> ASLGHPATFGRATHVVVRALPESLAQQALRRTKGDEVDFARAERQHQLYVGVLGSKLGLQVVQLPADESLPDCVFVEDVAVVCEETALITRPGAPSRRKEADMMKEALEKLQLNIVEMKDENATLDGGDVLFTGREF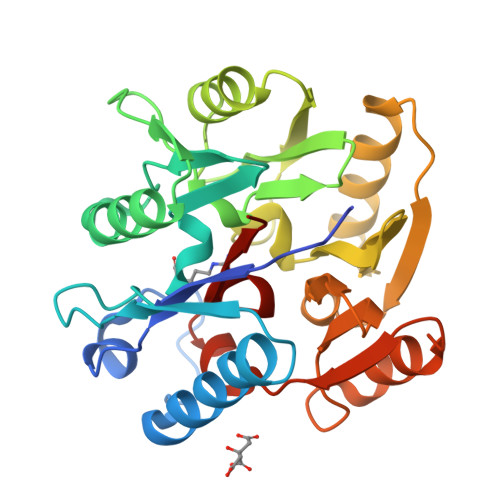FVGLSKRTNQRGAEILADTFKDYAVSTVPVVDALHLKSFCSMAGPNLIAIGSSESAQKALKIMQQMSDHRYDKLTVPDDTAANCIYLNIPSKGHVLLHRTPEEYPESAKVYEKLKDHMLIPVSNSELEKVDGLLTCSSVLINKKVDS>MPINKLRKRLGDLLVEEGIVSEAQLEQALNAQKNTGRRLGDTLISLGFLSETQLLN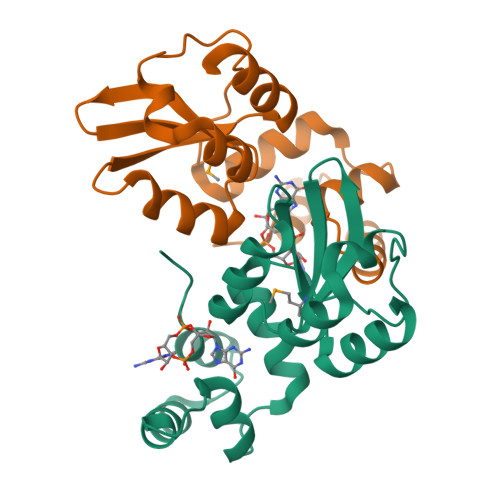FLAQQLSLPVIDLSRAHVDIDAVPLLPEVHARRLRALVIGRSGDTLRIAMSDPADLFAQEALLNQLPDYGFEFVIAPEKQLVDGFDRYY[2x]> MKQFGLAAFDELKDGKYNDVNKTILEKQSVELRDQLMVFQERLVEFAKKHNSELQASPEFRSKFMHMCSSIGIDPLSLFDRDKHLFTVNDFYYEVCLKVIEICRQTKDMNGGVISFQELEKVHFRKLNVGLDDLEKSIDMLKSLECFE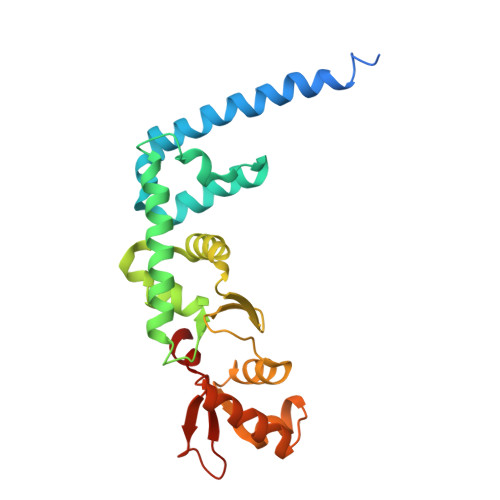IFQIRGKKFLRSVPNELTSDQTKILEICSILGYSSISLLKANLGWEAVRSKSALDEMVANGLLWIDYQGGAEALYWDPSWITRQL The cyclic oligonucleotide-based antiphage signalling system (CBASS) and the pyrimidine cyclase system for antiphage resistance (Pycsar) are antiphage defence systems in diverse bacteria that use cyclic nucleotide signals to induce cell death and prevent viral propagation. Here we show that phages encode anti-CBASS (Acb) and anti-Pycsar (Apyc) proteins that counteract defence by specifically degrading cyclic nucleotide signals that activate host immunity. Using a biochemical screen of 57 phages in Escherichia coli and Bacillus subtilis, we discover Acb1 from phage T4 and Apyc1 from phage SBSphiJ as founding members of distinct families of immune evasion proteins. We confirmed the critical role for Apyc1 metal-coordinating residues and identified E74 and Y112 from the opposing protomer as further catalytic residues required for cCMP hydrolysis and release of the reaction product 5′-CMP. Together, these findings demonstrate that Acb1 and Apyc1 constitute separate families of immune evasion proteins and explain the distinct reaction mechanisms that degrade CBASS or Pycsar cyclic nucleotide signals.

We next determined crystal structures of Acb1 to define the mechanism of anti-CBASS evasion. Structures of Acb1 from the Erwinia phage FBB1 in the apo state (1.1 Å) and in complex with 3′3′-cGAMP (1.2 Å) reveal that Acb1 adopts a compact 2H phosphoesterase fold with six central β-strands that form a U-shaped ligand-binding pocket. On substrate recognition, the flexible carboxy-terminal residues 145–152 form an ordered lid that closes over the top of the captured 3′3′-cGAMP ligand. Recombinant T4 Acb1 rapidly degrades the CBASS signals 3′3′-cGAMP, cUA and cAAA, but does not cleave cGG, demonstrating that Acb1 is responsible for the broad cyclic nucleotide hydrolysis activity observed in T4-infected cell lysate. The broad specificity of Acb1 allows evasion of diverse CBASS operons with a single gene, and the ability of Acb1 to cleave cyclic trinucleotide species suggests that this enzyme may also enable evasion of type III CRISPR systems that use cAAA signals.

> SGLYVAAKFSESTLDALEELQRSLKLPNPVPRDKLHTTIVYSRVNVPYKVASGSFEIADKGKLTVFETQSGNRALVLEMDSDYLSARHSYAKALGASYDYPDYRPHITLSYNIGVLNFSGEYKVPVVLDREYSEELDLEWSDKD>[2x]SKVTYIIKASNDVLNEKTATILITIAKK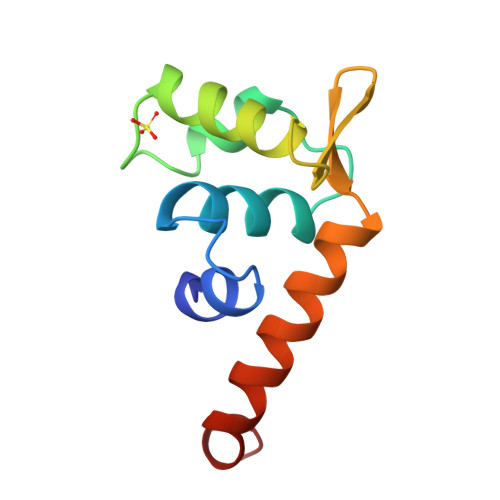DFITAAEVREVHPDLGNAVVNSNIGVLIKKGLVEKSGDGLIITGEAQDIISNAATLYAQENAPELLK> SMKNPEEEQKAKALRGRMFVLNELVQTEKDYVKDLGIVVEGFMKRIEEKGVPEDMRGKDKIVFGNIHQIYDWHKDFFLAELEKCIQEQDRLAQ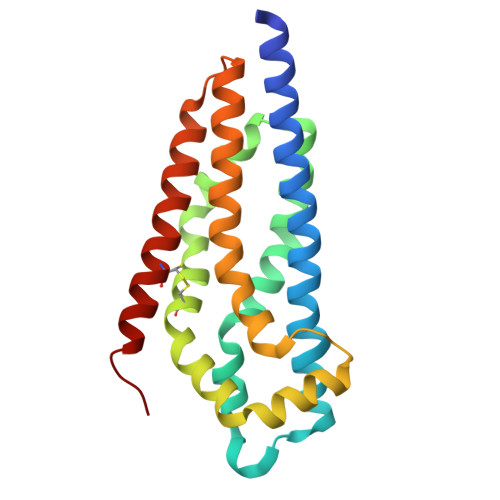LFIKHERKLHIYVWYCQNKPRSEYIVAEYDAYFEEVKQEINQRLTLSDFLIKPIQRITKYQLLLKDFLRYSEKAGLECSDIEKAVELMCLVPKRCNDMMNLGRLQGFE>GFPIPDPYCWDISFRTFYTIIDDEHKTLFNGILLLSQADNADHLNELRRCTGKHFLNEQQLMQSSQYAGYAEHKKAHDDF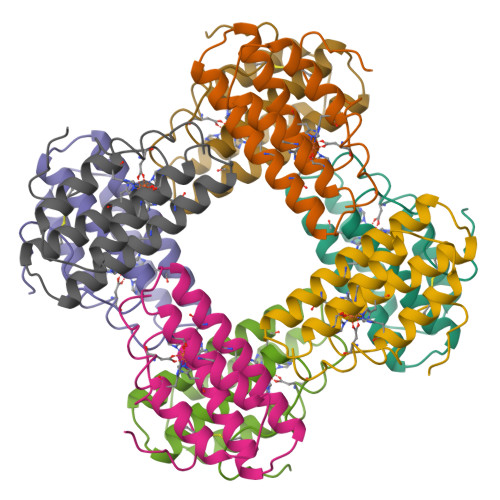IHKLDTWDGDVTYAKNWLVNHIKTIDFKYRGKI[4x]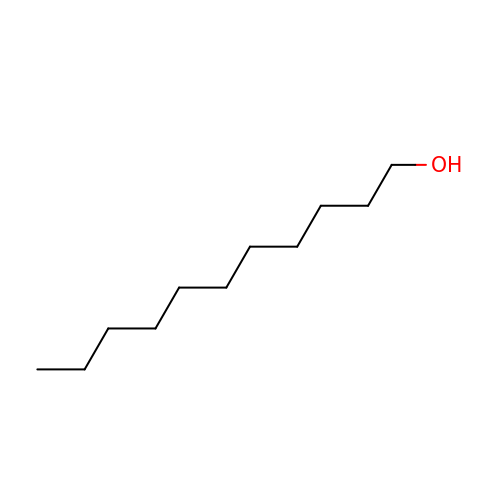undecan-1-ol | C11 H24 O | KJIOQYGWTQBHNH-UHFFFAOYSA-N>MLKKRGYDVTRNPHLNKGMAFTLEERLQLGIHGLIPPCFLSQDVQLLRIMRYYERQQSDLDKYIILMTLQDRNEKLFYRVLTSDVEKFMPIVYTPTVGLACQHYGLTFRRPRGLFITIHDKGHLATMLNSWPEDNIKAVVVTDGERILGLGDLGCYGMGIPVGKLALYTACGGVNPQQCLPVLLDVGTNNEELLRDPLYIGLKHQRVHGKAYDDLLDEFMQAVTDKFGINCLIQFEDFANANAFRLLNKYRNKYCMFNDDIQGTASVAVAGILAALRITKNKLSNHVFVFQGAGEAAMGIAHLLVMALEKEGVPKAEATRKIWMVDSKGLIVKGRSHLNHEKEMFAQDHPEVNSLEEVVRLVKPTAIIGVAAIAGAFTEQILRDMASFHERPIIFALSNPTSKAECTAEKCYRVTEGRGIFASGSPFKSVTLEDGKTFIPGQGNNAYVFPGVALGVIAGGIRHIPDEIFLLTAEQIAQEVSEQHLSQGRLYPPLSTIRDVSLRIAIKVLDYAYKHNL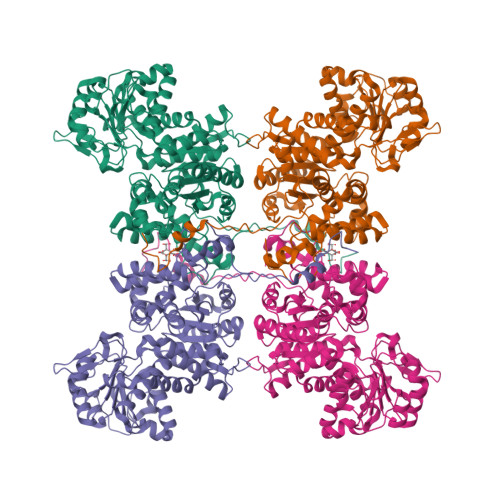ASYYPEPKDKEAFVRSLVYTPDYDSFTLDSYTWPKEAMNVQTVTRENLYFQ[2x]> MATT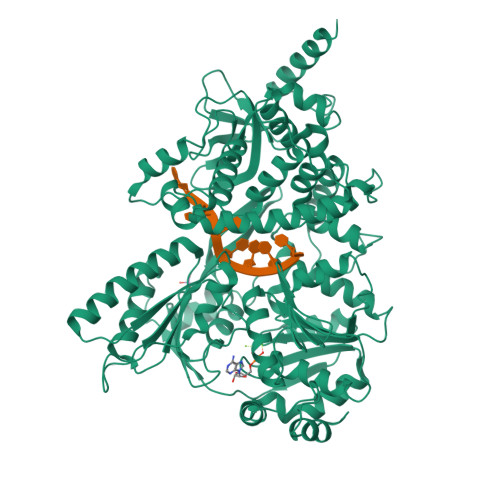AKQAEAVEDSDINPWTGQRHSERYFKILKARRKLPVNKQRQEFLDLYHNNQILVFVGETGSGKTTQIPQYVLYDELPHQTGKLIACTQPRRVAAMSVAQRVADELDVKLGEEVGYSIRFENKTSSKTLLKYMTDGQLLREAMHDRDMSRYSCIILDEAHERTLATDILMALLKQLSERRKDLKIIVMSATLDAQKFQSYFFNAPLLAVPGRTHPVEIFYTPEAERDYVEAAIRTVLQIHACEPEGDILLFLTGEEEIEDACRRISLEVDEMIRESDAGPMSVYPLYGTLPPHQQQRIFEKAPQPFRPGGRPGRKCIVATNIAETSLTIDGIVYVVDPGFSKQKIYNPRTRVESLLVSPISKASAQQRAGRAGRTRPGKCFRLYTEEAFKKELIEQTYPEILRSNLSNTVLELKKLGVEDLVHFDLMDPPAPETMMRALEELNYLACLDDDGELTPLGNLASEFPLDPALAVMLISSPEFYCSNEILSITSLLSVPQIWVRPANARKRADEMKAQFAHPDGDHLTLLNAYHAYKGAEARGEDMKKWCHEHFLSYRHLSSADNVRAQLKKIMETHGIELVSTPFHDKNYYTNIRRALLAGFFMQVAMRESSNSKVYKTVKDEQLVLIHPSTTVTTPYEWVVYNEFVLTTKQYVRTVTNIRPEWLLEIAPVYYDLSTFQKGEIKNALTRVAEKIRRQQAMKASKAWSHPQFEK>GTSMETFDPTELPELLKLYYRRLFPYSQYYRWLNYGGVIKNYFQHREFSFTLKDDIYIRYQSFNNQSDLEKEMQAANPYKIDIGAVYSHRPNQHNTVK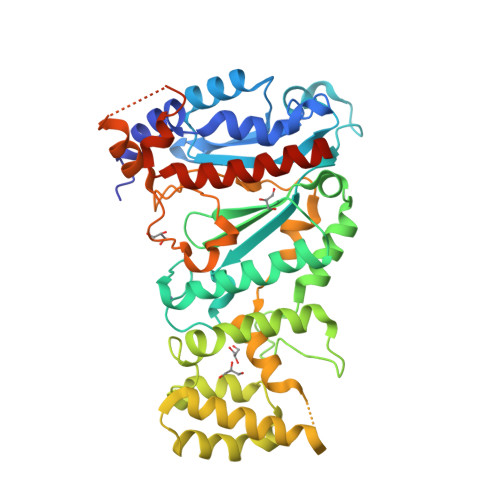LGAFQAQEKELVFDIDMTDYDDVRRCCSSADICPKCWTLMTMAIRIIDRALKEDFGFKHRLWVYSGRRGVHCWVCDESVRKLSSAVRSGIVEYLSLVKGGQDVKKKVHLSEKIHPFIRKSINIIKKYFEEYALVNQDILENKESWDKILALVPETIHDELQQSFQKSHNSLQRWEHLKKVASRYQNNIKNDKYGPWLEWEIMLQYCFPRLDINVSKGINHLLKSPFSVHPKTGRISVPIDLQKVDQFDPFTVPTISFICRELDAISTNEEEKEENEAESDVKHRTRDYKKTSLAPYVKVFEHFLENLDKSRKGELLKKSDLQKDF[2x];>[2x]MEFSGRKWRKLRLAGDQRNASYPHCLQFYLQPPSENISLIEFENLAIDRVKLLKSVENLGVSYVKGTEQYQSKLESELRKLKFSYRENLEDEYEPRRRDHISHFILRLAYCQSEELRRWFIQQEMDLLRFRFSILPKDKIQDFLKDSQLQFEAISDEEKTLREQEIVASSPSLSGLKLGFESIYKIPFADALDLFRGRKVYLEDGFAYVPLKDIVAIILNEFRAKLSKALALTARSLPAVQSDERLQPLLNHL> ADQPIDADVTVIGSGPGGYVAAIKAAQLGFKTVCIEKNETLGGTCLNVGCIPSKALLNNSHYYHMAHGKDFASRGIEMSEVRLNLDKMMEQKSTAVKALTGGIAHLFKQNKVVHVNGYGKITGKNQVTATKADGGTQVIDTKNILIATGSEVTPFPGITIDEDTIVSSTGALSLKKVPEKMVVIGAGVIGVELGSVWQRLGADVTAVEFLGHVGGVGIDMEISKNFQRILQKQGFKFKLNTKVTGATKKSDGKIDVSIEAASGGKAEVITCDVLLVCIGRRPFTKNLGLEELGIELDPRGRIPVNTRFQTKIPNIYAIGDVVAGPMLAHKAEDEGIICVEGMAGGAVHIDYNCVPSVIYTHPEVAWVGKSEEQLKEEGIEYKVGKFPFAANSRAKTNADTDGMVKILGQKSTDRVLGAHILGPGAGEMVNEAALALEYGASCEDIARVCHAHPTLSEAFREANLAASFGKS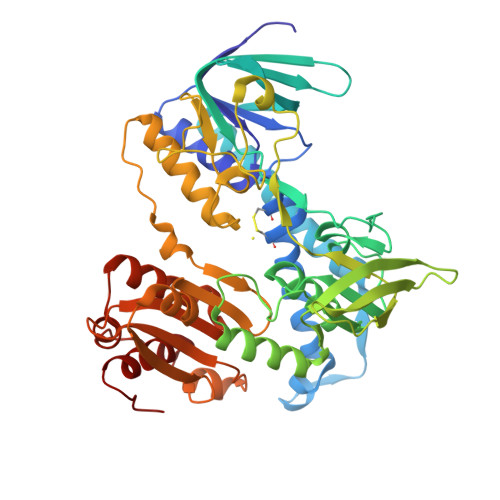INF>[4x]MGLALKKKSIPQPTNALKSFNWSKLPENKLEGTVWTEIDDTKVFKILDLEDLERTFSAYQRQQD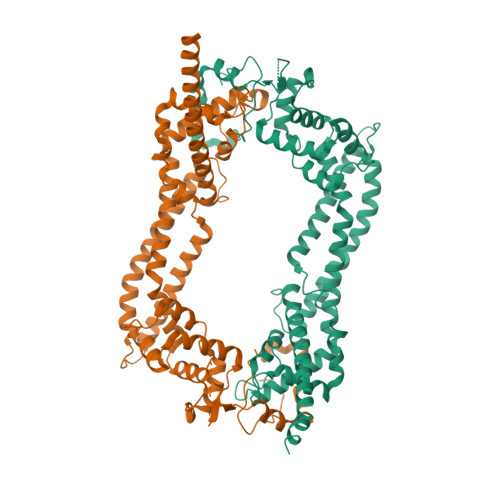FFVNSNSKQKEADAIDDTLSSKLKVKELSVIDGRRAQNCNILLSRLKLSNDEIKRAILTMDEQEDLPKDMLEQLLKFVPEKSDIDLLEEHKHELDRMAKADRFLFEMSRINHYQQRLQSLYFKKKFAERVAEVKPKVEAIRSGSEEVFRSGALKQLLEVVLAFGNYMNKGQRGNAYGFKISSLNKIADTKSSIDKNITLLHYLITIVENKYPSVLNLNEELRDIPQAAKVNMTELDKEISTLRSGLKAVETELEYQKSQPPQPGDKFVSVVSQFITVASFSFSDVEDLLAEAKDLFTKAVKHFGEEAGKIQPDEFFGIFDQFLQAVSEAKQENENMRKKKEEEERRARMEAQLKE> MSRRPWLLALALAVALAAGSAGASTGSDATVPVATQDGPDYVFHRAHERMLFQTSYTLENNGSVICIPNNGQCFCLAWLKSNGTNAEKLAANILQWITFALSALCLMFYGYQTWKSTCGWEEIYVATIEMIKFIIEYFHEFDEPAVIYSSNGNKTVWLRYAEWLLTCP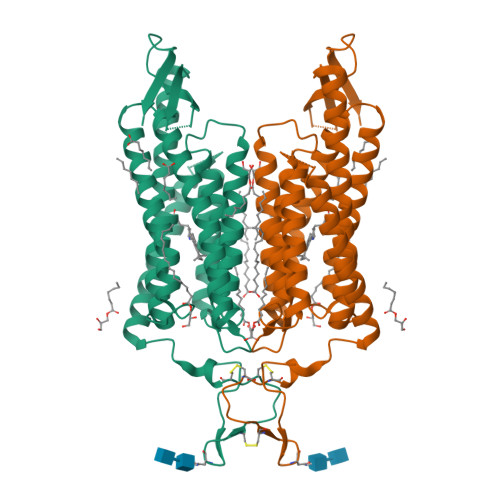VILIHLSNLTGLANDYNKRTMGLLVSDIGTIVWGTTAALSKGYVRVIFFLMGLCYGIYTFFNAAKVYIEAYHTVPKGRCRQVVTGMAWLFFVSWGMFPILFILGPEGFGVLSVYGSTVGHTIIDLMSKNCWGLLGHYLRVLIHEHILIHGDIRKTTKLNIGGTEIEVETLVEDEAEAGAVSSEDLYFQ> MKEFYLTVEQIGDSIFERYIDSNGRERTREVEYKPSLFAHCPESQATKYFDIYGKPCTRKLFANMRDASQWIKRMEDIGLEALGMDDFKLAYLSDTYNYEIKYDHTKIRVANFDIEVTSPDGFPEPSQAKHPIDAITHYDSIDDRFYVFDLLNSPYGNVEEWSIEIAAKLQEQGGDEVPSEIIDKIIYMPFDNEKELLMEYLNFWQQKTPVILTGWNVESFAIPYVYNRIKNIFGESTAKRLSPHRKTRVKVIENMYGSREIITLFGISVLDYIDLYKKFSFTNQPSYSLDYISEFELNVGKLKYDGPISKLRESNHQRYISYNIIAVYRVLQIDAKRQFINLSLDMGYYAKIQIQSVFSPIKTWDAIIFNSLKEQNKVIPQGRSHPVQPYPGAFVKEPIPNRYKYVMSFDLTSAYPSIIRQVNISPETIAGTFKVAPLHDYINAVAERPSDVYSCSPNGMMYYKDRDGVVPTEITKVFNQRKEHKGYMLAAQRNGEIIKEALHNPNLSVDEP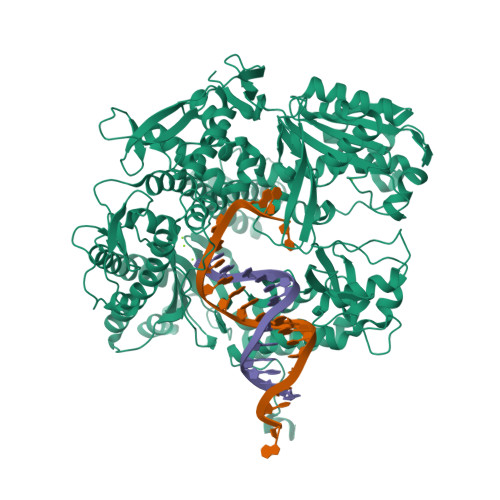LDVDYRFDFSDEIKEKIKKLSAKSLNEMLFRAQRTEVAGMTAQINRKALINGLAGALGNVWFRYYDLRNATAITTFGQMALQWIERKVNEYLNEVCGTEGEAFVLYGDTDSIYVSADKIIDKVGESKFRDTNHWVDFLDKFARERMEPAIDRGFREMCEYMNNKQHLMFMDREAIAGPPLGSKGIGGFWTGKKRYALNVWDMEGTRYAEPKLKIMGLETQKSSTPKAVQKALKECIRRMLQEGEESLQEYFKEFEKEFRQLNYISIASVSSANNIAKYDVGGFPGPKCPFHIRGILTYNRAIKGNIDAPQVVEGEKVYVLPLREGNPFGDKCIAWPSGTEITDLIKDDVLHWMDYTVLLEKTFIKPLEGFTSAAKLDYEKKASLFDMF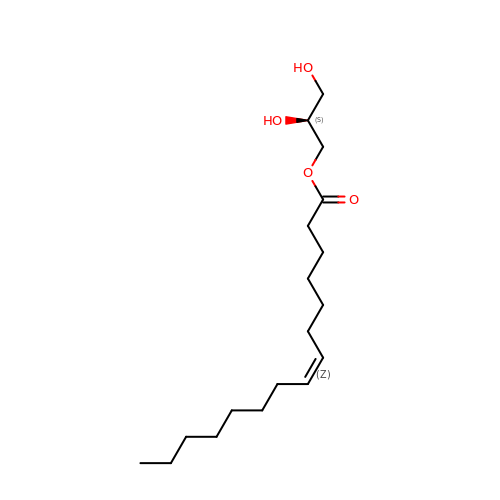(2S)-2,3-DIHYDROXYPROPYL(7Z)-PENTADEC-7-ENOATE | C18 H34 O4 | BJMLBVHMHXYQFS-JJEJIETFSA-N>DEKAAEVSELKLTKDNKEVVTLYANGNAFDKDGNQISSGTLTLTAKFKDQYGNELTGKVAGTDYTFESLNPEVLVVAPDGSVTPIVPGTALVKVKYGEVTKTIPVTVK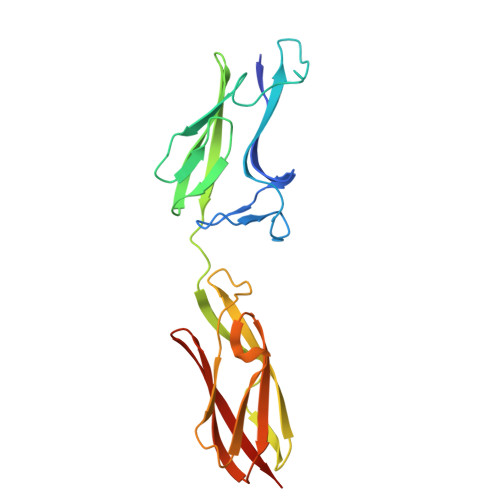ANPVLETIAVDSTGVSVAKGQKATFKVTLKDQYGNKFTGNVNVTSDKTETATVSVSNSGIGQSEYTVTVNGVAEGSTTITIKSGTKEVKVPVNVVAGGPV[2x]> ANKGFLEEVRKGNLERECLEEPCSREE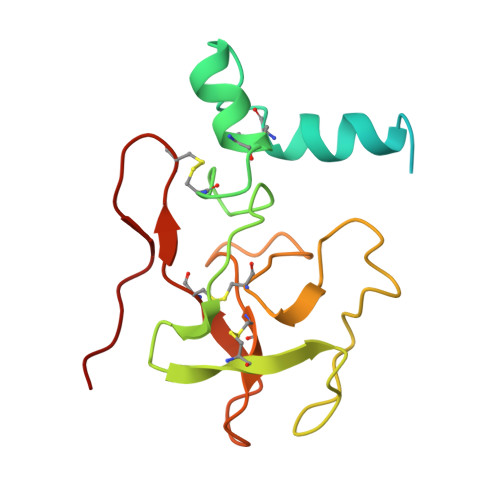AFEALESLSATDAFWAKYTACESARNPREKLNECLEGNCAEGVGMNYRGNVSVTRSGIECQLWRSRYPHKPEINSTTHPGADLRENFCRNPDGSITGPWCYTTSPTLRREECSVPVCGQDRVTVEVIPR>MATSFASRGGLLASGLAIAFWLTGCGTAEVTTSNAPSEEVTAVTTEVQGETEEKKKVLTTFTVLADMVQNVAGDKLVVESITRIGAEIHGYEPTPSDIVKAQDADLILYNGMNLEAWFEQFLGNVKDVPSVVLTEGIEPIPIADGPYTDKPNPHAWMSPRNALVYVENIRQAFVELDPDNAKYYNANAAVYSEQLKAIDRQLGADLEQVPANQRFLVSCEGAFSYLARDYGMEEIYMWPINAEQQFTPKQVQTVIEEVKTNNVPTIFCEST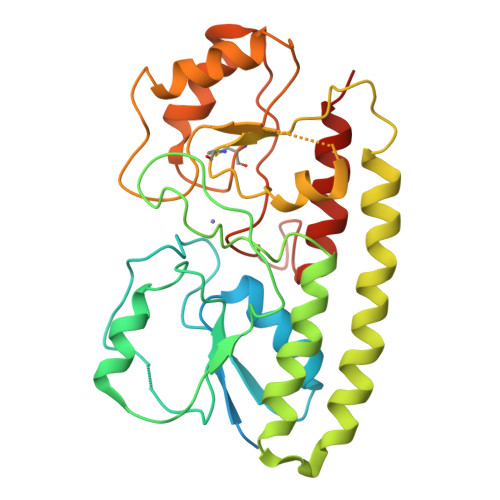VSDKGQKQVAQATGARFGGNLYVDSLSTEEGPVPTFLDLLEYDARVITNGLLAGTNAQQ[3x]>[2x]MGSSHHHHHH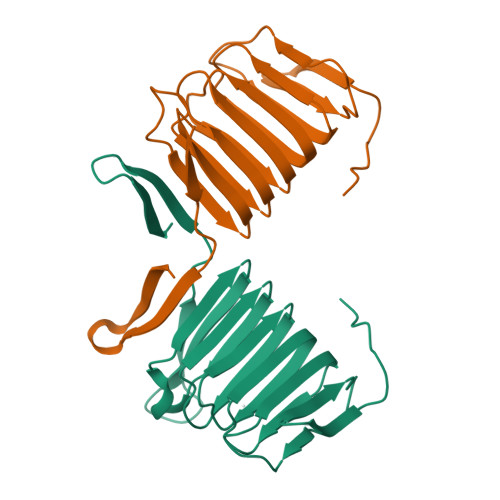SSGLVPRGSKSQIYLKKEKKMKAARQVVTNGSPKVELQKDTYLVENHVNCADPITLSEGSIKNKVSVRCSQNSRIIVEQKVNSIFIENCVGCIFLVNGVISSIEIVNCDDIKLQMTGIVPTISLDKSNKVNIYTSKEGKNVEVYSSKSSEMNLLFPGEEEGDWKELAIPEQFVTKYNESKGKLESMVSPLYG> METVISSDSSPAVENEHPQETPESNNSVYTSFMKSHRCYDLI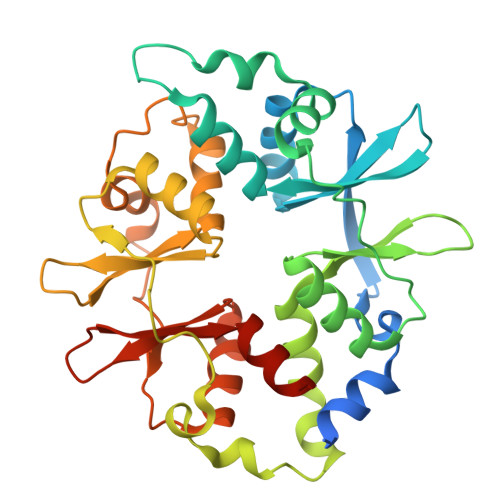PTSSKLVVFDTSLQVKKAFFALVTNGVRAAPLWDSKKQSFVGMLTITDFINILHRYYKSALVQIYELEEHKIETWREVYLQDSFKPLVCISPNASLFDAVSSLIRNKIHRLPVIDPESGNTLYILTHKRILKFLKLFITEFPKPEFMSKSLEELQIGTYANIAMVRTTTPVYVALGIFVQHRVSALPVVDEKGRVVDIYSKFDVINLAAEKTYNNLDVSVTKALQHRSHYFEGVLKCYLHETLETIINRLVEAEVHRLVVVDENDVVKGIVSLSDILQALVLTGGEKKP4-(4-phenoxy-1H-pyrazol-3-yl)benzene-1,3-diol 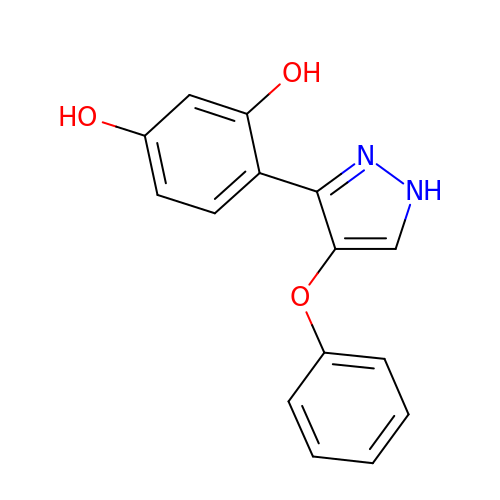| C15 H12 N2 O3 | WUNNLMRNOJZGQB-UHFFFAOYSA-N>MSDEQKKPEQIHRRDILKWGAMAGAAVAIGASGLGGLAPLVQTAAKPSKKDEKEEEQIVPFYGKHQAGITTAHQTYVYFAALDVTAKDKSDIITLFRNWTSLTQMLTSGKKMSAEQRNQYLPPQDTGESADLSPSNLTVTFGFGPGFFEKDGKDRFGLKSKKPKHLAALPAMPNDNLDEKQGGGDICIQVCADDEQVAFHALRNLLNQAVGTCEVRFVNKGFLSGGKNGETPRNLFGFKDGTGNQSTKDDTLMNSIVWIQSGEPDWMTGGTYMAFRKIKMFLEVWDRSSLKDQEDTFGRRKS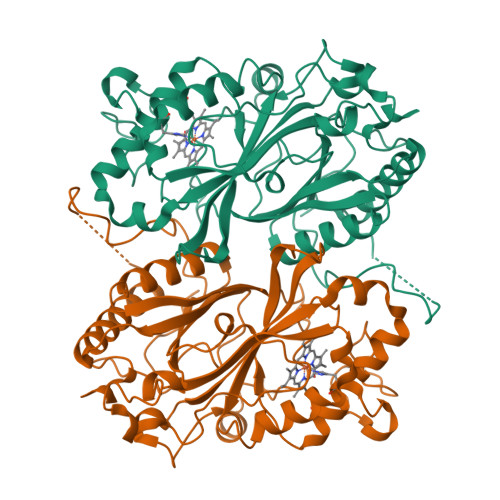SGAPFGQKKETDPVKLNQIPSNSHVSLAKSTGKQILRRAFSYTEGLDPKTGYMDAGLLFISFQKNPDNQFIPMLKALSAKDALNEYTQTIGSALYACPGGCKKGEYIAQRLLES[2x]> TSELRICRIDKESGPCTGGEELYLLCDKVQKEDISVRFSTASWEGRGDFSQADVHRQIAIVFKTPPYEDLEISEPVTVNVQLQRLTDGECSEPLPF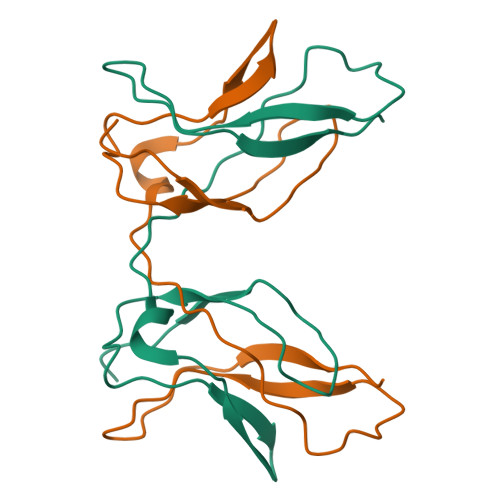TYLPR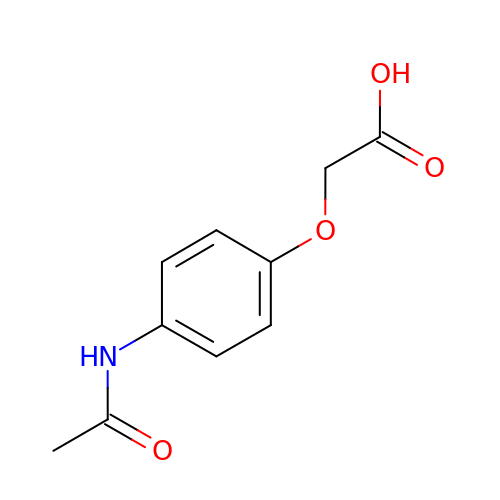2-(4-acetamidophenoxy)ethanoic acid | C10 H11 N O4 | LYJCGBYEVXKOST-UHFFFAOYSA-N>MPRPGHIAMVSVPSRGHLHPSLELIRELVARGHRVTYANDPSVAAAVTETGAELVPYTSALPSTDTTEGRVTDQIAQMDVFLDDAVGMLPQLRAAYEEDRPDVFLYDVLAYPARVLAMNWGIPSIQISPTWVMPEKYRERMAPVVEQLKQDPRGAAHYRRFDAWLEDSGVPGIDAGDLVNLPERSLVLVPRFLQPDADDVDEKRFTFIGPCLGRRAHQGDWKRPAGAEKVALVSLGSHLTNQLPFYETCVEVFAALPDWHLVLQIGRHVDAGELGELPPNVEVHNWVPQLAVLEQADVFVTHGGMGGIQEGLFSGVPMVVAPQANDQPANAESVV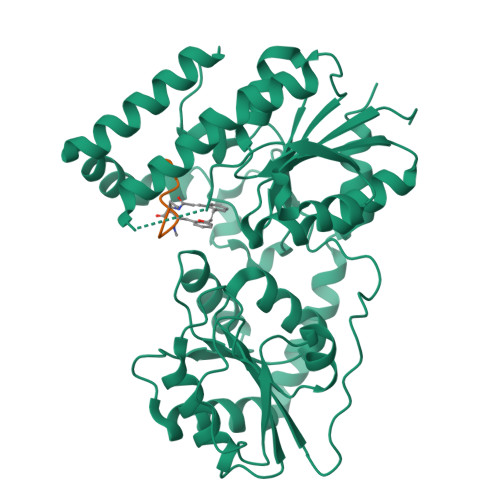GLGIARRIDIATVTPDRLRAAVVELASDPAVAERLSGLRRELRAHGGTMRAADLIERQLPA[4x];>[4x]XNVFVGGVL>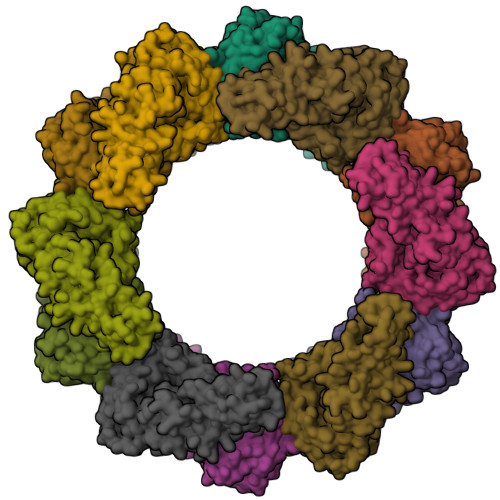[12x]MSTLKNTFFITPPDTPTQAGPENIFYDFNDGARVLLPEGKWHVRLLDADSENILFCCDVDKGWVTSSKKYFVRFRIQVFRQGEETPLLDETLKLKDRPVLISFPTGTLGALLGWFPYAERFQSLHKCRLECTMSQDIIDLLAPQYPQIQFSTPDKPRTVAPYATYRVGLYFGGDTNNQPVDFRKVGFHRSAGYILGVDPREAPVRLDLSAPRVIQEPYVCIATQSTCQAKYWNNGTGWSEVIAHLKSLGYRVMCIDRDAHYGQGFVWNHIPWGAEDFTGKLPLQERVNLLRHASFFIGLPSGLSWLAWATRIPVVLISGFSLPNSEFYTPWRVFNSHGCYGCWDDTSLNFDHHDFLWCPRHKNTDRQFECTRLITGAQVNGVINKLHRSLTEQGVEATLKKGVSNE> GPLGSWSWESYLEEQKAITAPVSLFQDSQAVTHNKNGFKLGMKLEGIDPQHPSMYFILTVAEVCGYRLRLHFD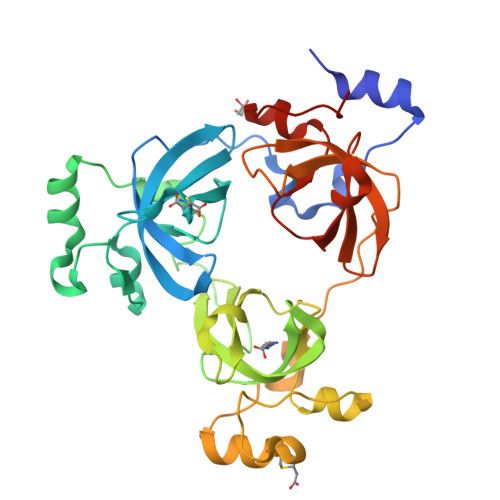GYSECHDFWVNANSPDIHPAGWFEKTGHKLQPPKGYKEEEFSWSQYLRSTRAQAAPKHLFVSQSHSPPPLGFQVGMKLEAVDRMNPSLVCVASVTDVVDSRFLVHFDNWDDTYDYWCDPSSPYIHPVGWCQKQGKPLTPPQDYPDPDNFCWEKYLEETGASAVPTWAFKVRPPHSFLVNMKLEAVDRRNPALIRVASVEDVEDHRIKIHFDGWSHGYDFWIDADHPDIHPAGWCSKTGHPLQPPLG>MGSDKIHHHHHHMMVISEKVRKALNDQLNREIYSSYLYLSMATYFDAEGFKGFAHWMKKQAQEELTHAMKFYEYIYERGGRVELEAIEKPPSNWNGIKDAFEAALKHEEFVTQSIYNILELASEEKDHATVSFLKWFV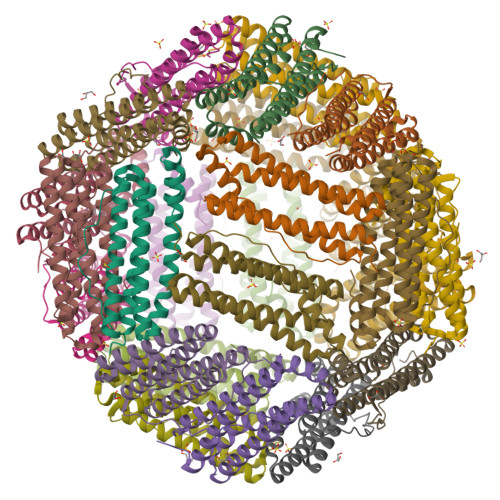DEQVEEEDQVREILDLLEKANGQMSVIFQLDRYLGQRE[8x]>[6x]SNAMTIKGRAFPEGFLWGGAVAAHQLEGGYKEGGKGLSTADIMTLGTNERPREITDGVVAGKYYPNHQAIDFYHRYPEDIELFAEMGFKCFRTSIAWTRIFPNGDESEPNEAGLQFYDDLFDECLKNGIQPVVTLAHFEMPYHLVKQYGGWRNRKLIQFYLNFAKVCFERYRDKVTYWMTFNEINNQTNFESDGAMLTDSGIIHQPGENRERWMYQAAHYELVASAAAVQLGHQINPDFQIGCMIAMCPIYPLTAAPADVLFAQRAMQTRFYFADVHCNGTYPQWLRNRFESEHFNLDITAEDLKILQAGTVDYIGFSYYMSFTVKDTGKLAYNEEHDLVKNPYVKASDWGWQVDPVGLRYAMNWFTDRYHLPLFIVENGLGAIDKKTADNQIHDDYRIDYLTDHLRQIKLAVLEDGVDLIGYTPWGCIDLVAASTGQMSKRYGFIYVDENDDGSGSLKRYKKDSFTWFQHVIATNGAEIE

Specifically, the β-­glycosidic bond of 6′-P-β-glucoside is cleaved by 6-P-β-glucosidase (6PβGlu; EC 3.2.1.86), releasing 6-P-β-glucose (BG6; glycon), an important cellular precursor, and the remaining portion of the given substrate (aglycon). Here, the high-resolution crystal structures of GH1 6-P-β-glucosidases from Lactobacillus plantarum (LpPbg1) and Streptococcus mutans (SmBgl) and their complexes with ligands are reported. 6PβGlu is a single-domain protein that adopts a (β/α)8-barrel (TIM-barrel) structure, which is a typical fold of GH1-family members. The GH1-family enzymes utilize a double-displacement mechanism of catalysis with retention of configuration at the anomeric C atom of the glycon moiety.

The LpPbg1 structure has been determined in an apo form as well as in a complex with phosphate and a glucose molecule corresponding to the aglycon molecule. The apo form of LpPbg1 was solved in the trigonal space group P31 with six protein chains in the asymmetric unit, 547 water molecules, one glycerol molecule and six chloride ions. The refined atomic model included residues Ala0–Glu478 of chains A and D, Thr2–Ala334 and Gln350–Glu478 of chain B, Thr2–Asp346 and Gly348–Glu478 of chain C, Met1–Leu42, Arg49–Ala344 and Gln350–Glu478 of chain E and Met1–Thr44, Pro48–Lys343 and Gln350–Glu478 of chain F. The crystals are merohedrally twinned with twin operator k, h, −l and a refined twin fraction of 0.28. Superposition of LpPbg1 with apo LpPbg1 yields an r.m.s.d. of between 0.42 and 0.65 Å (for chains B and F, respectively).> MGSDKIHHHHHHMFPYKIVDDVVILMPNKELNIENAHLFKKWVFDEFLNKGYNKIFLVLSDVESIDSFS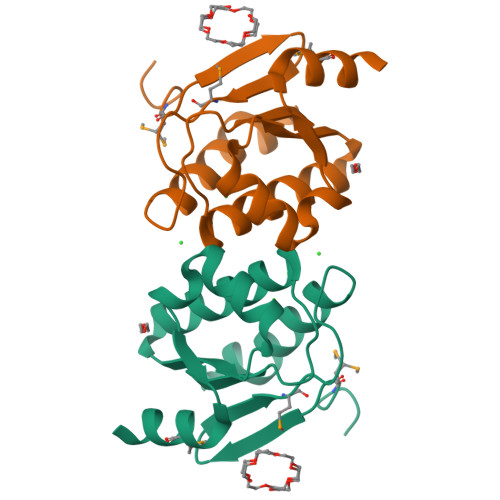LGVIVNILKSISSSGGFFALVSPNEKVERVLSLTNLDRIVKIYDTISEAMEEVRRK>VDLEKIPIEEVFQQLKCSREGLTTQEGEDRIQIFGPNKLEEKKESKLLKFLGFMWNPLSWVMEMAAIMAIALANGDGRPPDWQDFVGIICLLVINSTISFIEENNAGNAAAALMAGLAPKTKVLRDGKWSEQEAAILVPGDIVSIKLGDIIPADARLLEGDPLKVDQSALTGESLPVTKHPGQEVFSGSTCKQGEIEAVVIATGVHTFFGKAAHLVDSTNQVGHFQKVLTAIGNFCICSIAIGMVIEIIVMYPIQRRKYRDGIDNLLVLLIGGIPIAMPTVLSVTMAIGSHRLSQQGAITKRMTAIEEMAGMDVLCSDKTGTLTLNKLSVDKNLVEVFCKGVEKDQVLLFAAMASRVENQDAIDAAMVGMLADPKEARAGIREVHFLPFNPVDKRTALTYIDGSGNWHRVSKGAPEQILELAKASNDLSKKVLSIIDKYAERGLRSLAVARQVVPEKTKESPGAPWEFVGLLPLFDPPRHDSAETIRRALNLGVNVKMITGDQLAIGKETGRRLGMGTNMYPSSALLGTHKDANLASIPVEELIEKADGFAGVFPEHKYEIVKKLQERKHIVGMTGDGVNDAPALKKADIGIAVADATDAARGASDIVLTEPGLSVIISAVLTSRAIFQRMKNYTIYAVSITIRIVFGFMLIALIWEFDFSAFMVLIIAILNDGTIMTISKDRVKPSPTPDSWKLKEIFATGVVLGGYQAIMTVIFFWAAHKTDFFSDTFGVRSIRDNNHELMGAVYLQVSIISQALIFVTRSRSWSFVERPGALLMIAFLIAQLIATLIAVYANWEFAKIRGIGWGWAGVIWLYSIVTYFPLDVFKFAIRYI[2x]

The Arabidopsis thaliana plasma membrane H+-ATPase 2 (AHA2) is a member of the PIII-subtype of the P-type ATPase superfamily. It pumps protons out of the cell to maintain a steep electrochemical H+ gradient and potential across the plasma membrane. Structural organization of AHA2 encompasses a cytoplasmic headpiece formed by three domains; the nucleotide (N) binding domain, the phosphorylation (P) domain, and the actuator (A) domain, as well as a membrane domain composed of 10 transmembrane segments harboring the proton binding site and the translocation pathway (Pedersen et al., 2007). Additionally and similar to other members of the PIII subfamily, AHA2 has N- and C-terminal extensions involved in auto-regulatory functions, the latter being considerably longer and referred to as the R-domain.

Here, we have made use of new model-building and refinement tools to present a new, re-refined atomic model of AHA2, which can be employed for more accurate structural comparisons and models of transport. Rebuilding and re-refinement employed the new interactive molecular dynamics flexible fitting (iMDFF) approach in combination with phenix.refine and resulted in a significantly improved model with new features emerging in the electron density maps. The application of iMDFF environment in refinement of low-resolution protein structures was successfully reported in studies on Human Insulin Receptor Ectodomain, and we have applied it here to the original, highly anisotropic 3.6 Å resolution crystallographic data obtained from AHA2 crystals. Structural changes of the revised AHA2 model includes a local rearrangement of transmembrane helices 7 and 8, where ~1-turn N-terminal register shift is observed, and local changes at the nucleotide binding pocket of the N-domain. Additionally, improvement in the model quality allowed for inclusion of a conserved K+-binding site located at the P-domain. The proton translocation pathway, which centers on earlier identified residues Asn106, Asp684, and Arg655, begins at the cytoplasmic side of the TM domain from where protons are delivered to the Asn-Asp pair via a solvent tunnel located between TM1, 2, 4, and 6. Solvent accessibility of the proton entrance is obtained by a characteristically short, helical structure of TM1. Based on modeling of E1P-E2P conformational changes, protons are likely transported via a large solvent-filled cavity that merges with an exit pathway toward the extracellular side of the membrane. Arg655, proximal to the cavity stimulates deprotonation of Asp684 and proton release, serving as a built-in counter ion required for E2P closure and dephosphorylation and the E2-E1 transition of the pump. The AHA2 structure reveals mechanistic concepts that can also be recognized in other transmembrane proton/cation transport systems, yet future structures of E2 states will be required to fully elucidate functional transitions of PIII-type H+-ATPases.2-{[5-CHLORO-2-({(1E,4R)-2-METHOXY-4-[(3R)-3-(METHYLAMINO)PYRROLIDIN-1-YL]CYCLOHEXA-2,5-DIEN-1-YLIDENE}AMINO)PYRIMIDIN-4-YL]AMINO}-N-(1-METHYLETHYL)BENZENESULFONAMIDE 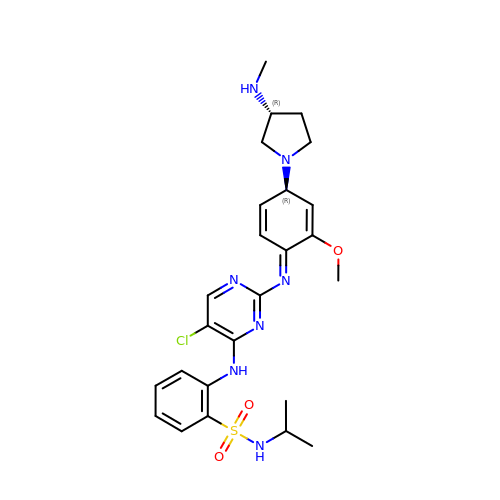| C25 H32 Cl N7 O3 S | GLVPQZCTTHRANR-ZYGFWXSESA-N> MASIDAFSDLERRMDGFQKDVAQVLARQQNHVALYERLLQLRVLPGASDVHDVRFVFGDDSRCWIEVAMHGDHVIGNSHPALDPKSRATLEHVLTVQGDLAAFLVV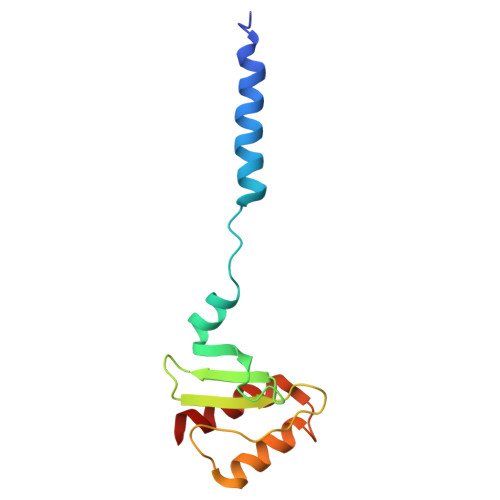ARDMLLAS>[2x]SKTKPFSLPILTLSELTNSRFPVPIDSLFT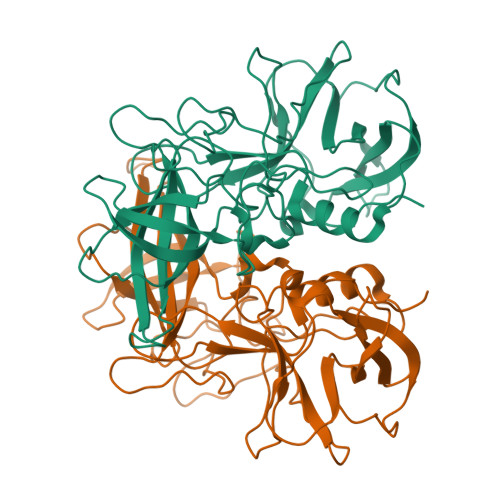AQNNVLQVQCQNGRCTLDGELQGTTQLLPSGICAFRGRVTAQINQRDRWHMQLQNLNGTTYDPTDDVPAPLGTPDFKGVVFGMVSQRNVGNDAPGSTRAQQAWVSTYSPQFVPKLGSVNLRISDNDDFQFQPTKFTPVGVNDDDDGHPFRQWELPNYSGELTLNMNLAPPVAPNFPGEQLLFFRSFVPCSGGYNQGIIDCLIPQEWIQHFYQESAPSQSDVALIRYVNPDTGRTLFEAKLHRSGYITVAHSGDYPLVVPANGHFRFDSWVNQFYSLAPM> MQASQFSAQVLDWYDKYGRKTLPWQIDKTPYKVWLSEVMLQQTQVATVIPYFERFMARF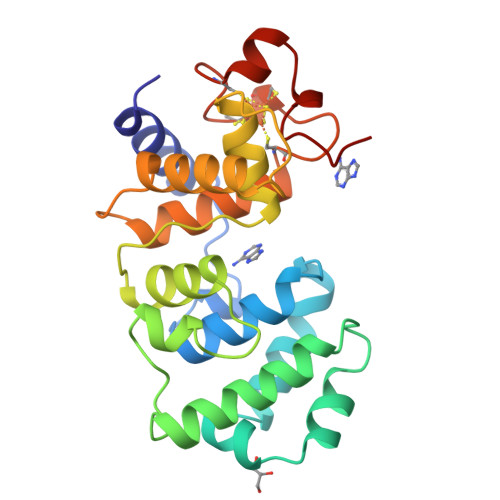PTVTDLANAPLDEVLHLWTGLGYYARARNLHKAAQQVATLHGGKFPETFEEVAALPGVGRSTAGAILSLSLGKHFPILNGNVKRVLARCYAVSGWPGKKEVENKLWSLSEQVTPAVGVERFNQAMMDLGAMICTRSKPKCSLCPLQNGCIAAANNSWALYPGKKPK> SS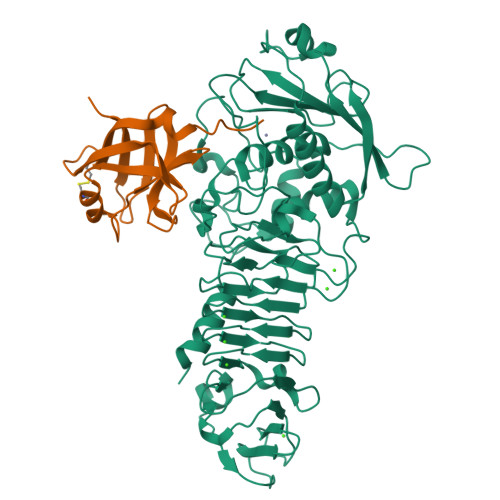LILLSASDLAGQWTLQQDEAPAICHLELRDSEVAEASGYDLGGDTACLTRWLPSEPRAWRPTPAGIALLERGGLTLMLLGRQGEGDYRVQKGDGGQLVLRRATP;> GRSDAYTQVDNFLHAYARGGDELVNGHPSYTVDQAAEQILREQASWQKAPGDSVLTLSYSFLTKPNDFFNTPWKYVSDIYSLGKFSAFSAQQQAQAKLSLQSWSDVTNIHFVDAGQGDQGDLTFGNFSSSVGGAAFAFLPDVPDALKGQSWYLINSSYSANVNPANGNYGRQTLTHEIGHTLGLSHPGDYNAGEGDPTYADATYAEDTRAYSVMSYWEEQNTGQDFKGAYSSAPLLDDIAAIQKLYGANLTTRTGDTVYGFNSNTERDFYSATSSSSKLVFSVWDAGGNDTLDFSGFSQNQKINLNEKALSDVGGLKGNVSIAAGVTVENAIGGSGSDLLIGNDVANVLKGGAGNDILYGGLGADQLWGGAGADTFVYGDIAESSAAAPDTLRDFVSGQDKIDLSGLDAFVNGGLVLQYVDAFAGKAGQAILSYDAASKAGSLAIDFSGDAHADFAINLIGQATQADIVV>MRGSHHHHHHGSMRKPIIGVMGPGEQATPTDLKNAYQLGQLIALEGWVLLTGGRNVGVMEHASQGAKKAEGLTIGILPSKNTHNVSDAVDIAIVTGLGNARNNINVLSSDVVIACGIG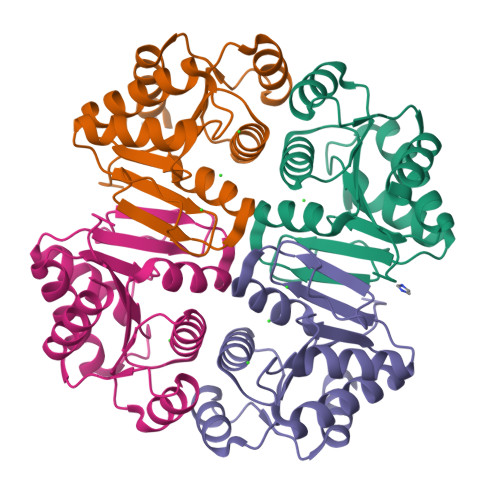LGTLSEVALALKNQKPVILLNDDLLSQELFANLSNNQVWIASSPENCIELIKSIITVKLN[4x]>GFKQDIATIRGDLRTYAQDIFLAFLNKYPDERRNFKNYVGKSDQELKSMAKFGDHTEKVFNLMMEVADRATDCVPLASDANTLVQMKQHSGLTTGNFEKLFVALVEY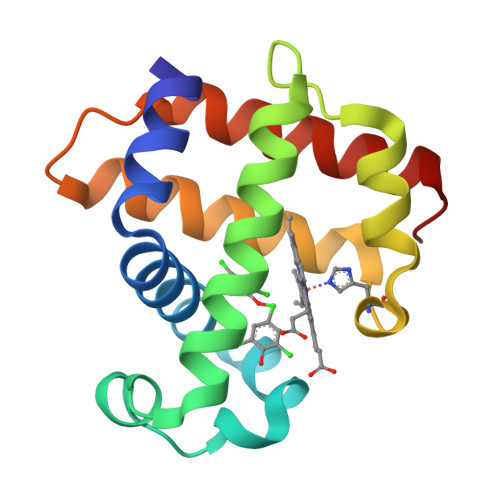MRASGQSFDSQSWDRFGKNLVSALSSAGMK[2x]Mimivirus is the prototype of the Mimiviridae family of giant dsDNA viruses. Little is known about the organization of the 1.2 Mb genome inside the membrane-limited nucleoid filling the ~0.5 µm icosahedral capsids. Cryo-electron microscopy, cryo-electron tomography, and proteomics revealed that it is encased into a ~30-nm diameter helical protein shell surprisingly composed of two GMC-type oxidoreductases, which also form the glycosylated fibrils decorating the capsid. The genome is arranged in 5- or 6-start left-handed super-helices, with each DNA-strand lining the central channel.

Finally, the 4-Å resolution Cl2 map obtained after 3D refinement corresponds to a 6-start left-handed helix made of a~8-nm-thick proteinaceous external shell, with six dsDNA strands lining the shell interior and leaving a ~12-nm-wide inner channel. Compared to Cl1a, the Cl2 6-start helix (G) shows a difference of ~2° relative to the fiber longitudinal axis and ~2° in the steepness of the helical rise. Further, some intermediate and relaxed structures were also observed in which the DNA segments appeared detached from the protein shell and sometimes completely absent from the central channel of the broken fibers. Both GMC oxidoreductases (qu_946 and qu_143) can be fitted in the 5- and 6-start maps. In the Cl1a and Cl2 helices, the monomers in each dimer are interacting with two different dsDNA strands. As a result, the DNA strands are interspersed between two dimers, each also corresponding to a different strand of the protein shell helix. Density that can be attributed to the FAD cofactor is also present in the Cl2 and Cl3a maps.

>MKNRECCKCYNPCEKICVNYSTTDVAFERPNPCKPTPCKPTPIPCDPCHNTKDNLTGDIVIIGAGAAGSLLAHYLARFSNMKIILLEAGHSHFNDPVVTDPMGFFGKYNPPNENISMSQNPSYSWQGAQEPNTGAYGNRPIIAHGMGFGGSTMINRLNLVVGGRTVFDNDWPVGWKYDDVKNYFRRVLVDINPVRDNTKASITSVALDALRIIAEQQIASGEPVDFLLNKATGNVPNVEKTTPDAVPLNLNDYEGVNSVVAFSSFYMGVNQLSDGNYIRKYAGNTYLNRNYVDENGRGIGKFSGLRVVSDAVVDRIIFKGNRAVGVNYIDREGIMHYVKVNKEVVVTSGAFYTPTILQRSGIGDFTYLSSIGVKNLVYNNPLVGTGLKNHYSPVTITRVHGEPSEVSRFLSNMAANPTNMGFKGLAELGFHRLDPNKPANANTVTYRKYQLMMTAGVGIPAEQQYLSGLSPSSNNLFTLIADDIRFAPEGYIKIGTPNIPRDVPKIFFNTFVTYTPTSAPADQQWPIAQKTLAPLISALLGYDIIYQTLISMNQTARDSGFQVSLEMVYPLNDLIYKLHNGLATYGANWWHYFVPTLVGDDTPAGREFADTLSKLSYYPRVGAHLDSHQGCSCSIGRTVDSNLKVIGTQNVRVADLSAAAFPPGGNTWATASMIGARAVDLILGFPYLRDLPVNDVPILNVN[2x]>[4x]GSLHCPAACTCSNNIV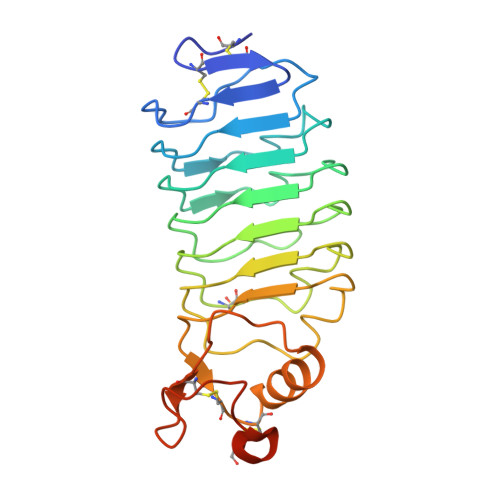DCRGKGLTEIPTNLPETITEIRLEQNTIKVIPPGAFSPYKKLRRIDLSNNQISELAPDAFQGLRSLNSLVLYGNKITELPKSLFEGLFSLQLLLLNANKINCLRVDAFQDLHNLNLLSLYDNKLQTIAKGTFSPLRAIQTMHLAQNPFICDCHLKWLADYLHTNPIETSGARCTSPRRLANKRIGQIKSKKFRCSAAAHHHHHH(2~{R},3~{S},4~{R},5~{R},6~{R})-5-azanyl-2-(hydroxymethyl)-6-(4-naphthalen-2-yl-1~{H}-imidazol-2-yl)oxane-3,4-diol 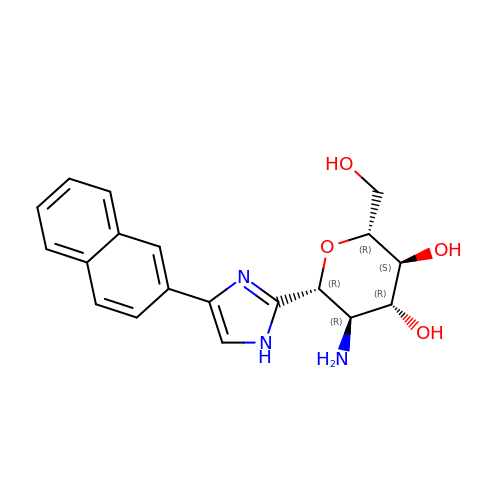| C19 H21 N3 O4 | VXVNVASERGBQNT-DUQPFJRNSA-N In Pseudomonas aeruginosa, Ttg2D is the soluble periplasmic phospholipid-binding component of an ABC transport system thought to be involved in maintaining the asymmetry of the outer membrane. Sequence analysis indicates that Ttg2DPae (PA4453) is the soluble periplasmic SBP component of the ABC transporter encoded by the ttg2 operon and a member of the Pfam family MlaC (PF05494). Thus, we present structural and functional evidence of the role of this protein as a general phospholipid transporter capable of carrying either diacyl or tetra-acyl glycerophospholipids. The soluble substrate-binding protein Ttg2DPae, together with the inner membrane complex Ttg2ABCE, transports mislocalised glycerophospholipids between the two cell membranes through the periplasm of P. aeruginosa.

Here we use the crystallographic structure of Ttg2D at 2.5 Å resolution to reveal that this protein can accommodate four acyl chains. Ttg2DPae adopts a mixed α + β fold with a highly twisted anti-parallel β-sheet formed by five strands and surrounded by eight α-helices. It exhibits a “decanter” shaped structure never described before for any other protein family. The structure presents a highly hydrophobic cavity between the β-sheet and the helices that spans the whole protein and has a volume of 2979 Å3 and a depth of ~25 Å. After the first refinement stage (AutoBuild), without any ligand added, clear density was visible inside the cavity that could correspond to four acyl chains. We therefore modeled inside the cavity two PG(16:0/cy17:0), as mass spectrometry (MS) experiments suggested that this lipid was one of the most abundant among those found to bind Ttg2DPae when expressed in E. coli (see below). The four acyl tails are deeply inserted into the hydrophobic cavity, while the polar head groups are exposed to the solvent and make only few contacts with the protein. This lack of specific recognition of the head group could explain why Ttg2DPae is able to bind different types of phospholipids. Indeed, for the second group (R. solanacearum and E. coli, one diacyl lipid), this helix has a straight conformation, covers the α6 helix and does not participate in the cavity, while in the first group (P. aeruginosa and P. putida, two diacyl lipids), the α8 helix is bent towards and over the α7 helix and greatly enlarges the cavity (with additional residues from β4 and β5 strands).

> MAPTPQQVVQGTVDELLSDIKANKAAYKADPQKLYATLDRILGPVVDAEGIAKSVMTVKYSRQASPEQIKRFEEVFKNSLMQFYGNALLEYDNQDIRVLPSSAKPSDDRASVNMEIRDSKGTVYPVSYTMTNLAGGWKVRNVIINGINIGKLFRDQFADTMQKNRNDLEKTIAGWGEVVAKAKETAKAEEAGAKKLAAALEHHHHHH>MGGSHHHHHHGDDDDKMTKTFKTLDDFLGTHFIYTFDNGWEY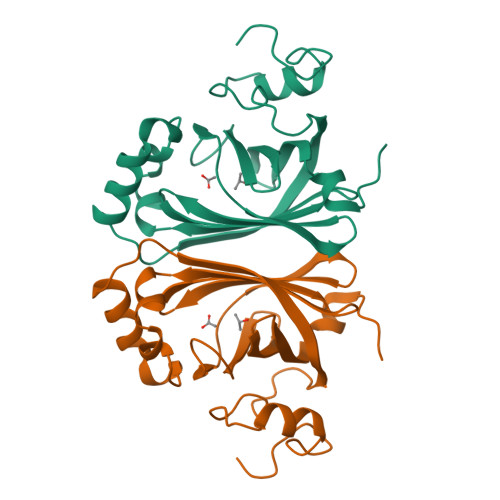EWYAKNDHTVDYRIHGGMVAGRWVTDQKADIVMLTEGIYKISWTEPTGTDVALDFMPNEKKLHGTIFFPKWVEEHPEITVTYQNEHIDLMEQSREKYATYPKLVVPEFANITYMGDAGQNNEDVISEAPYKEMPNDIRNGKYFDQNYHRLNK[2x]>[2x]MNKVVLLCRPGFEKECAAEITDKAGQREIFGFARVKENAGYVIYECYQPDDGDKLIRELPFSSLIFARQWFVVGELLQHLPPEDRITPIVGMLQGVVEKGGELRVEVA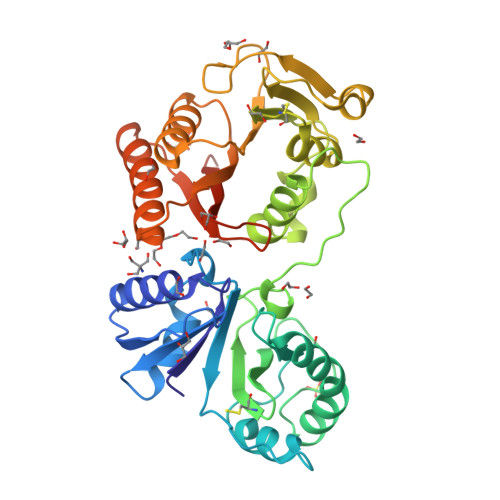DTNESKELLKFCRKFTVPLRAALRDAGVLANYETPKRPVVHVFFIAPGCCYTGYSYSNNNSPFYMGIPRLKFPADAPSRSTLKLEEAFHVFIPADEWDERLANGMWAVDLGACPGGWTYQLVKRNMWVYSVDNGPMAQSLMDTGQVTWLREDGFKFRPTRSNISWMVCDMVEKPAKVAALMAQWLVNGWCRETIFNLKLPMKKRYEEVSHNLAYIQAQLDEHGINAQIQARQLYHDREEVTVHVRRIWAAVGGRRDERSKGHHHHHH> DKATIPS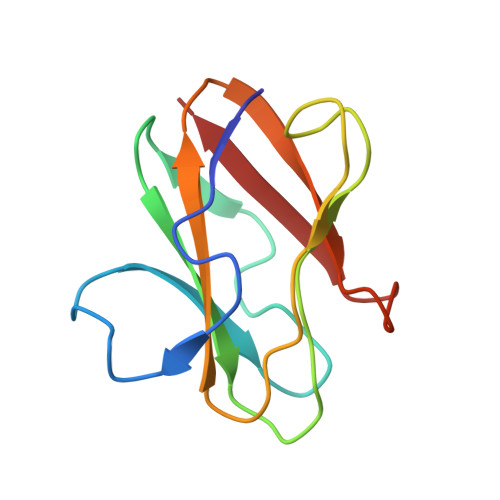ESPFAAAEVADGAIVVDIAKMKYETPELHVKVGDTVTWINREAMPHNVHFVAGVLGEAALKGPMMKKEQAYSLTFTEAGTYDYHCTPHPFMRGKVVVE> MLYILNSAILPLKPGEEYTVKAKEITIQEAKELVTKEQFTSAIGHQATAELLSSILGVNVPMNRVQIKVTHGDRILAFMLKQRLPEGVVVKTTEELEKIGYELWLFEIQ

AFV3-109 is the most conserved protein in different families of crenarchaeal viruses. The structure of AFV3-109 is a five stranded β-sheet with loops on one side and three helices on the other. It forms a dimer adopting the shape of a cradle that encompasses the best conserved regions of the sequence. Although the function of AFV3-109 cannot be deduced directly from its structure, structural homology with the STIV1 protein, and the size and charge distribution of the cavity suggested it could interact with nucleic acids.

The protein was crystallized in two different space groups, C2221 and P3121, depending on the pH of the mother liquor (pH 8.8 and 4.0, respectively). The structures were solved at 1.5 (C2221) and 1.3 Å (P3121) resolution. Crystals of both space groups contain a single copy of the protein in the asymmetric unit. Both structures are almost identical with a r.m.s. deviation between both crystal forms of 0.5Å for all Cα positions. Strengthening this argument, identical dimers could be formed from symmetry related molecules in both crystal forms. An r.m.s. deviation of 0.51 Å is observed for all Cα atoms of the two dimers. The second (2 residues) is in the tip of the long connection between β4 and β5 and is juxtaposed to the best conserved sequence region (see further). This large conformational difference in the connection between β4 and β5 with B116 is obeyed for the two crystal forms of AFV3-109 who superpose perfectly in this region. The refinement of the C2221 crystal structure identified the presence of a strong residual electron density in the cavity, in close contact with the His45 side-chain. We modelled this density as a glycerol molecule, present in the mother liquid as crystal cryoprotectant. In contrast, a glycerol molecule could not fit into a residual density present near His45 in the P3121 space group.> GPEPDMISVFIGTWNMGSVPPPKNVTSWFTSKGLGKTLDEVTVTIPHDIYVFGTQENSVGDREWLDLLRGGLKELTDLDYRPIAMQSLWNIKVAVLVKPEHENRISHVSTSSVKTGIANTLGNKGAVGVSFMFNGTSFGFVNCHLTSGNEKTARRNQNYLDILRLLSLGDRQLNADDISDRFTHLFWFGDLNYRLDMDIQEILNYISRKEFEPLLRVDQLNLEREKHKVFLRFSEEEISFPPTYRYERGSRDTYAWHKQKPTGVRTNVPSWCDRILWKSYPETHIICNSYGCTDDIVTSDHSPVFGTFEVGVTSQFISKKGLSKTSDQAYIEFESIEAIVKTASRTKFFIEFYSTCLEEYKKSFENDAQSSDNINFLKVQWSSRQLPTLKPILADIEYLQDQHLLLTVKSMDGYESYGECVVALKSMIGSTAQQFLTFLSHRGEETGNIRGSMKVRVPTER

The two main enzymes responsible for PI(3,4,5)P3 degradation are the tumor suppressor phosphatase and tensin homolog (PTEN), which removes the 3-phosphate (3 P) and the SH2-containing inositol 5-phosphatase (SHIP), which dephosphorylates the 5 P to generate PI(3,4)P2. The SHIP Ptase domain belongs to a family of Mg2+-dependent inositol phosphatases with specificity for 5 P dephosphorylation of inositol rings. Here, we report the crystal structure of SHIP2 containing the 5-Ptase and a C2 domain (Ptase-C2), revealing that the two domains tightly associate via an extensive interface. Importantly, even in the absence of a localization effect, the C2 domain provides activating signals to the Ptase active site, resulting in a significant increase in catalytic turnover.

In order to disrupt the hydrophobic core of the domain interface we mutated F593 and L597 to aspartates (FLDD mutant). Crystal structures of Ptase-C2 FLDD confirm that few hydrophobic interactions remain intact between the Ptase and C2 domains. The FLDD mutations also disrupt interdomain hydrogen bonds between R649 and E862. When comparing the catalytic turnover of the FLDD mutants we find that the C2 domain no longer has a significant effect with either substrate, indicating that the FLDD mutations largely mimic the absence of the C2 domain. We note that the FLDD mutations increase intrinsic Ptase activity with PI(3,4,5)P3-diC8, but importantly the presence of the C2 does not cause any further change. The PS-mediated increase in activity on vesicles is maintained for the FLDD mutant, whereas as with soluble substrates, the increase in activity due to the C2 domain is abrogated by the interface mutations. Removing the C2 domain abolishes observed SHIP2 activity, whereas the FLDD mutations partially reduce activity of the wild-type protein.> MVQQKVEVRLKTGLQARP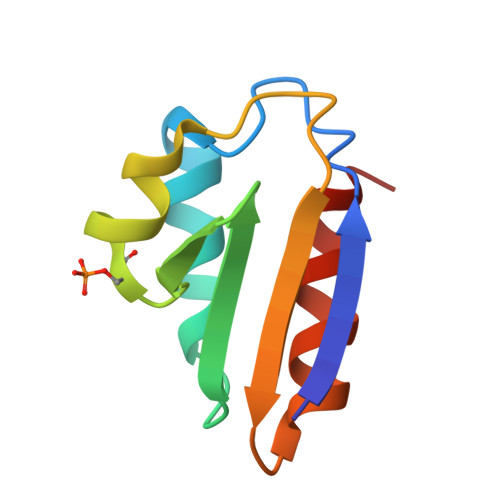AALFVQEANRFTSDIFLEKDGKKVNAKSIMGLMSLAISTGTEITLIAQGEDEQEALEKLAAYVQEEV>MHHHHHHMPIIEQVRAREILDSRGNPTVEVEVALIDGTFARAAVPSGASTGEHEAVELRDGGDRYGGKGVQKAVQAVLDEIGPAVIGLNADDQRLVDQALVDLDGTPDKSRLGGNAILGVSLAVAKAAADSAELPLFRYVGGPNAHILPVPMMNILNGGAHADTAVDIQEFMVAPIGAPSFVEALRWGAEVYHALKSVLKKEGLSTGLGDEGGFAPDVAGTTAALDLISRAIESAGLRPGADVALALDAAATEFFTDGTGYVFEGTTRTADQMTEFYAGLLGAYPLVSIEDPLSEDDWDGWAALTASIGDRVQIVGDDIFVTNPERLEEGIERGVANALLVKVNQIGTLTETLDAVTLAHHGGYRTMISHRSGETED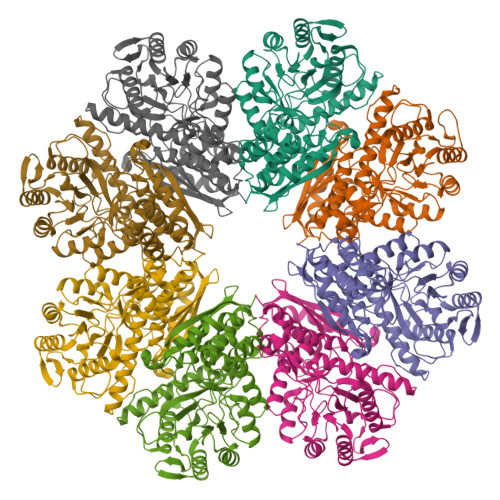TMIADLAVAIGSGQIKTGAPARSERVAKYNQLLRIEEALGDAARYAGDLAFPRFACETK[8x]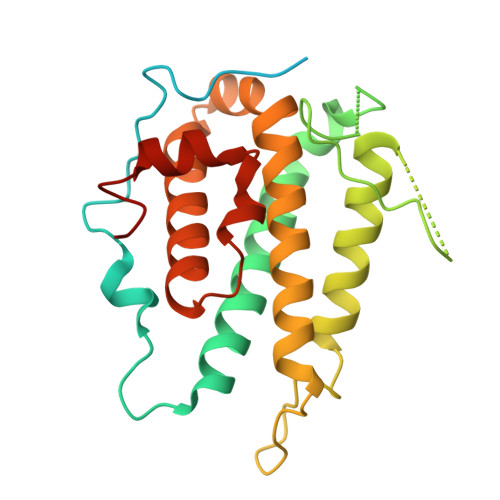> GSLRNKHHSPKRHSQTSFPAQKSTPQSQQLTSTTPQSQQQEASERSESQQIMFLSEPFVRTALVKGSFKTIVQLPKYVDLGEWIALNVFEFFTNLNQFYGVVAEYCTPDACPTMNAGPHTDYLWLDANNRQVSLPASQYIDLALTWINNKVNDKNLFPTKNGLPFPQQFSRDVQRIMVQMFRIFAHIYHHHFDKIVHLSLEAHWNSFFSHFISFAKEFKIIDRKEMAPLLPLIESFEKQGKIIYN> FQSMMLDRIRVVLVNTSHPGNIGGAARAMKNMGLSQLVLVQPESFPHGDAVARASGATDILDAAR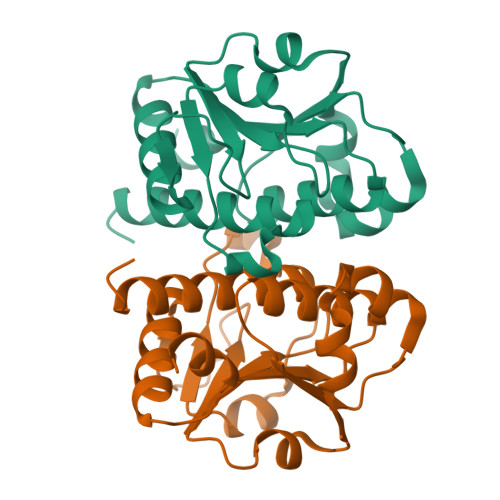VVDTLEEALSGCSVVLGTSARDRRIPWPLLDPRECATTCLEHLEANGEVALVFGREYAGLTNEELQRCQFHVHIPSDPEFGSLNLAAAVQVLTYEVRMAWLAAQGK> SMDRRFYGKIVIKGKIKAVTGLHIGSQRDISEIGGIANPVIKDPHTGLPYI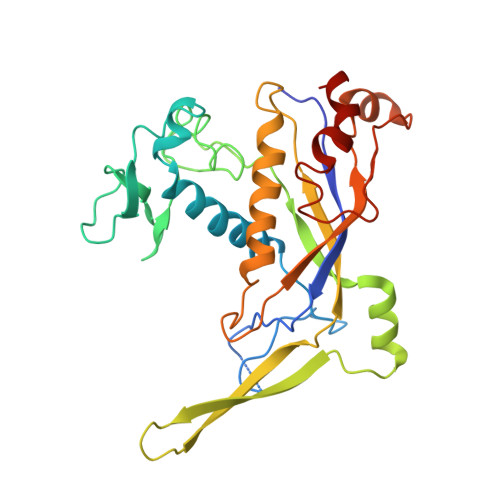PGSSLKGRLRSLFEILVNSRLGEWREKYPSLANYSPGSCRPDNQENCGKFFNRKINRGWIHVCPDYETALACPVCRLFGASGKESNFPSRIIVRDAFLTKEWEEKWRAGEAITEAKIEVGIDRVTSQANPRTNERVVAGAEFEFEIIYNVENTTHWRDDIKNLLTAMALLEDSYLGGSGSRGYGKVKFIFDSFEFRPLDYYRTGKDEDIVSIDAREKSVSDILSGFDSLFSEVEGKLEAG> MNDIAHNLAQVRDKISAAATRCGRSPEEITLLAVSATAPASAIAEAIDAGQRQFGENYVQEGVDKIRHFQELGVTGLEWHFIGPLQSNKSRLVAEHFDWCHTIDRLRIATRLNDQRPAELPPLNVLIQINISDENSKSGIQLAELDELAAAVAE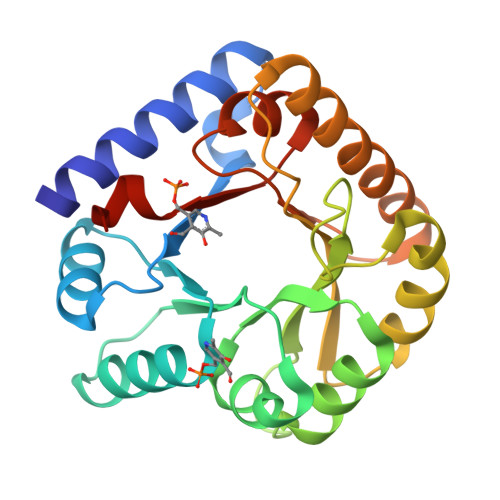LPRLRLRGLMAIPAPESEYVRQFEVARQMAVAFAGLKTRYPHIDTLSLGMSDDMEAAIAAGSTMVRIGTAIFGARDYSAA[(4-{[(4S)-2,7-diphenylimidazo[1,2-a]pyridin-3-yl]amino}phenyl)methyl]phosphonic acid | C26 H22 N3 O3 P | 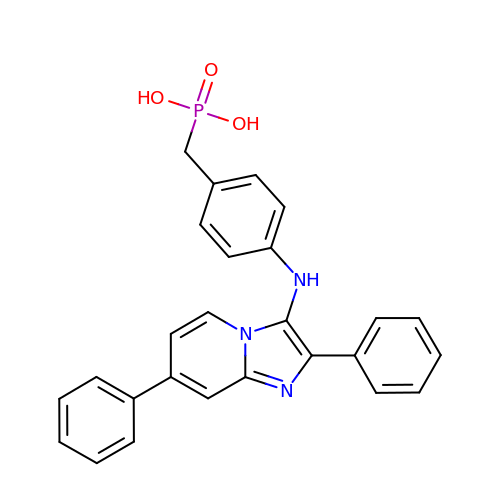ORMINEGKRFWUKK-UHFFFAOYSA-N Recently, RNF112 has emerged as an intriguing addition to the dynamin-like large GTPase superfamily, which has been widely implicated in mediating biological membrane remodeling events, including membrane tubulation, fission, and fusion. To obtain an architectural overview of RNF112, we carried out structural studies on modified Xenopus laevis RNF112 constructs in different nucleotide-loading states. For these constructs (collectively denoted as RNF112T), the N-terminal RING domain, the predicted transmembrane helix, and the C-terminal amphipathic helix were removed. RNF112T is composed of a GTPase domain (GD) and a middle domain (MD) comprising a 3-helix bundle.

Nucleotide-free RNF112T contains several disordered regions in the nucleotide-binding site in the GD, involving all G1-G4 motifs, which take up as much as ~15% of the total GD in terms of the number of amino acid residues. Thus, the disordered G1 motif of RNF112 in the nucleotide-free state makes it unique in the dynamin superfamily, representing an extremely flexible catalytic center before binding nucleotides. However, nucleotide-free RNF112T and RNF112T-GDP form 2 adopt a unique conformation that has never been observed with ATLs. The MD of nucleotide-free RNF112T stays perpendicular to α8G and swings ~30° from the position of GDP•AlF4−-bound RNF112T MD when the GDs are superimposed. Compared to the GDP•AlF4−-bound form, the Hinge 2 loop in nucleotide-free RNF112T involutes toward the GD from the outstretching conformation, leading to an ~90° rotation around the long axis of the MD. Importantly, the GD also exhibited local conformational changes at the backside of the nucleotide-binding pocket, involving redirection of helix α4G and relocation of the loop between α7G and α8G, which creates a big groove to dock the MD. Accompanied by the wedging of the MD into this groove are extensive interdomain contacts. Met456, Met458, Phe459, and Ile462 from the MD; Phe452 and Pro455 from the Hinge 2 loop; and Ile280, Ala284, Tyr308, Met311, Met315, Phe441, Val444, and Leu445 from the GD form a massive intramolecular hydrophobic network. Therefore, the interdomain contacts are unique to nucleotide-free RNF112 and stabilize its specific conformation. Given the similarities with other dynamin superfamily members, a special structural feature of RNF112 is seen at its nucleotide-free state, which is characterized by a 30° rigid-body swing of the MD relative to the GD and a new intramolecular interface between the two domains.

> AEPDHPIQLVWTDVNGRLSLDLSGAHDCFLNTRYSNYPVFILCIIGEKRRGKSFLMNYIMRALRSMEMDEEISLGADDEPLKGFKWSPGTETTTKGIWMWNRPFLLNHKGGKIAVFLLDTEGSLDIESDRETCIKLSALSLFISSHLIFNVASNLKETELDYMEMYMNMGEECGPKNLQHLDILVRDWYHSKKWDRDVARSYISREIEKLEKLNSYPKVLWSLKSNQTRCFLLPHPGKGITGESEGRLQDMDEDFQESLRSYVSKVVKGICTHIKTNIDGELLTSAHVFSMLQEFTEVLNLQIYGFSSPMEMFYAIKNQKLMGEIENEFQDFLKNQSSLTLPPTMRVKVSQKFSELLEKFMQFVQGSNTSSHDAMLKDLEVRLLEIQEKFCNDFTTRFT>MGHHHHHHAENLYFQGADPFESYNPEFFLYDIFLKFCLKYIDGEICHDLFLLLGKYNILPYDTSNDSIYACTNIKHLDFINPFGVAAGFDKNGVCIDSILKLGFSFIEIGTITPRGQTGNAKPRIFRDVESRSIINSCGFNNMGCDKVTENLILFRKRQEEDKLLSKHIVGVSIGKNKDTVNIVDDLKYCINKIGRYADYIAINVSSPNTPGLRDNQEAGKLKNIILSVKEEIDNLEKNNIMNDESTYNEDNKIVEKKNNFNKNNSHMMKDAKDNFLWFNTTKKKPLVFVKLAPDLNQEQKKEIADVLLETNIDGMII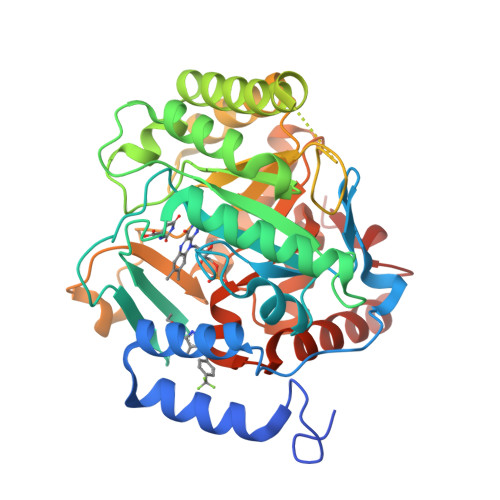SNTTTQINDIKSFENKKGGVSGAKLKDISTKFICEMYNYTNKQIPIIASGGIFSGLDALEKIEAGASVCQLYSCLVFNGMKSAVQIKRELNHLLYQRGYYNLKEAIGRKHSKS[4x]> LDYHACGGRLTDDYG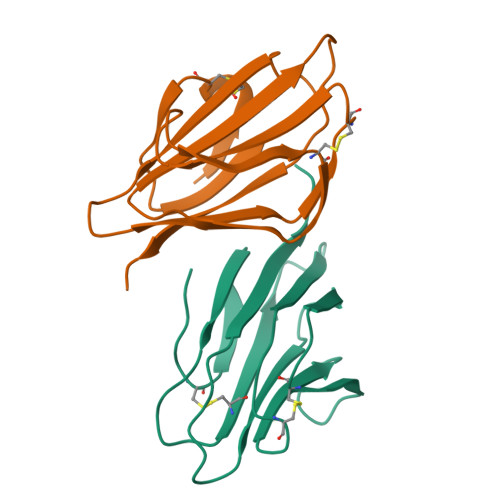TIFTYKGPKTECVWTLQVDPKYKLLVSIPTLNLTCGKEYVEVLEGAPGSKSLGKFCEGLSILNRGSSGMTVKYKRDSGHPASPYEIIFLRDSQG;> ARINGPDECGRVIKDTSGSISNTDRQKNLCTWTILMKPDQKVRMAIPYLNLACGKEYVEVFDGLLSGPSYGKLCAGAAIVFLSTANTMTIKYNRISGNSSSPFLIYFYGSSPGSEY>[2x]MNTLSPRLRKAMNTAAWAHRHHVRKGGGIPYVSHLYSVMYLLASVTNDEDVLIAGLLHDTLEDVPEEYNSAQLEADFGPRVRELVEELTKQPLKSWKARADAYLLHLSAGASLEA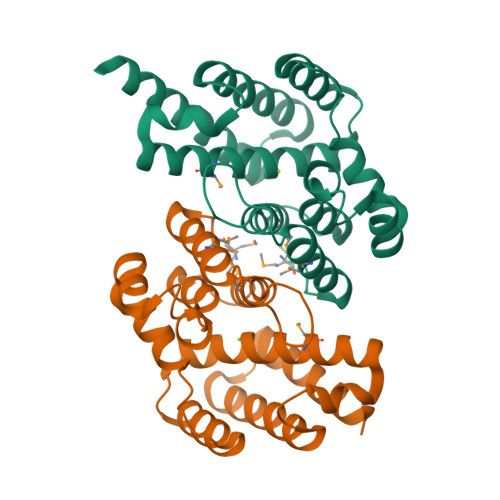VLISTADKLHNLMSILDDLEIHGEDLWQRFNAGKEQQIWWYSEVYQISLQRLGFNELNKQLGLCVEKLLKQSALEHHHHHH>MTMQGFGVHTSMWTMNWDRPGAERAVAAALKYEVDFIEIPMLNPPAVDTEHTRALLEKNELRALCSLGLPERAWASVRPDAAIEHLKVAIDKTADLGGEALSGVIYGGIGERTGVPPTEAEYDNIARVLSAAAKHAKSRGIELGVEAVNRYENHLINTGWQAVQMIERVGADNIFVHLDTYHMNIEEKGVGNGILDAREHLKYIHLSESDRGTPGYGTCGWDEIFSTLAAIGFKGGLAMESFINMPPEVAYGLAVWRPVAKDEEEV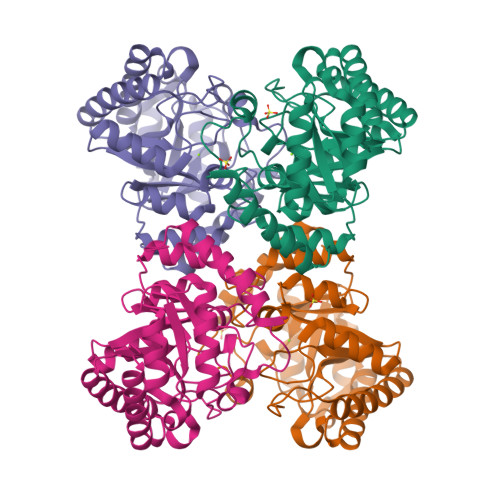MGNGLPFLRNKAKQYGLIGN[4x]BENZENE-1,2,3,4-TETRAYL TETRAKIS[DIHYDROGEN (PHOSPHATE)] | C6 H10 O16 P4 | 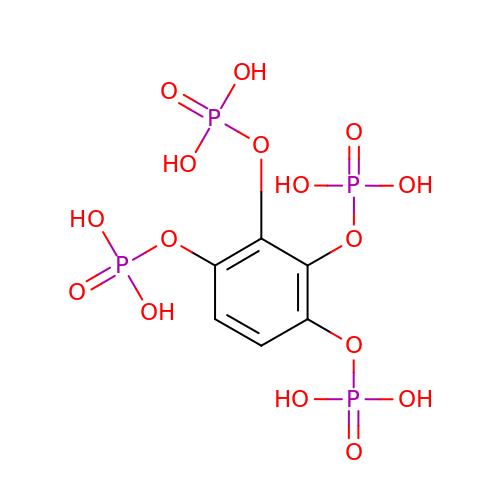UKRGHRHHBNLNDD-UHFFFAOYSA-N> SENSLEIEELARFAVDEHNKK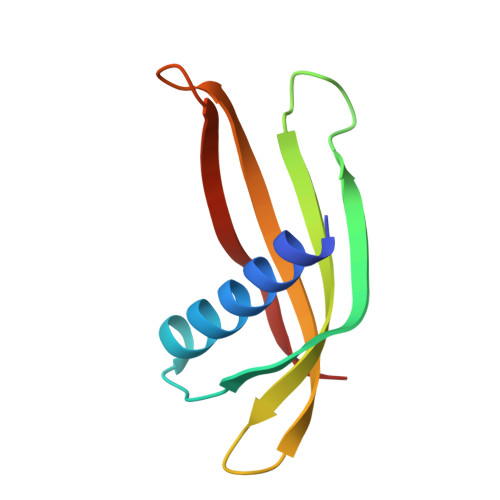ENALLEFVRVVKAKEQMGVNPEEMQTMYYLTLEAKDGGKKKLYEAKVWVKWWWGFHIWDNFKELQEFKPV> MSETQSQTMTRPQDLSLSDINSTVEVPEGHSFWKTLLAYSGPGALVAVGYMDPGNWSTSITGGQNFQYLLLSIIVISSLLAMLLQNMAAKLGIVCQLDLAQAIRARTSRRLGFIFWILTELAIMATDIAEVIGAAIALYLLFKIPIFLAVVITVLDVFLLLLLNRIGFRKIEALVVCLIFVILFVFLYQIILSQPAWHQVAKGLIPSWASVQTSPKIGGQTPLSASLGIIGATIMPANLFLHSAISQSRKIDRTDSSKVAEAVRFSNWDSNIQLSLAMVVNALLLIMGVAVFKSGAVQDPSFFGLYQALSNPDMVSNPVLAEAARSGVLSTLFAVALLASGQNSTITGTITGQVIMEGFIHLRLPLWLRRLVTRLIAIIPVVVCVAITSHQGSLDEHQALNNLMNNSQVFLALALPFSIVPLLMLTDSAAQMGNQFKNTRWVKVMGWLTVIILTLLNLISISSQIAGFFGDNPSSQDLLLSQVISIGIILAMIGLLIWTIIDIRRFTHPKQKALEVLFQ

conserved and function as secondary active transporters. transport proteins that include the amino acid transporter LeuT18. μM range and that metal ion transport is coupled to the cotransport of protons. of the prokaryotic SLC11 transporter EcoDMT.

mutants of Glu129 and reduced to half in H236A. different role in proton-coupled metal ion transport. residual H+ transport that may have escaped our detection.We previously determined the crystal structure of the C-terminal 73-residue fragment of PhBCCP (PhBCCPΔN76) that represents the biotinyl(/lipoyl attachment) domain of the hypothetical methylmalonyl-CoA decarboxylase γ chain. This domain adopts a flattened β-barrel comprising two homologous ‘hammerhead’ structures that confer an intramolecular pseudo-twofold symmetry reflecting the gene duplication. In this work, we used the C-terminal 70-residue fragment of PhBCCP (PhBCCPΔN79) as the template to prevent the N-terminal heterogeneity that was observed in PhBCCPΔN76. Moderate deviations of up to 2.53 Å were observed at residues 114–116, which constitute a flexible β-turn harbouring the Lys115 residue to be biotinylated.

In the PhBCCP system (PhBCCPΔN79) residue 138 was selected as the target residue for the mutation experiment because it is a solvent-exposed and nonconserved residue on a surface β-sheet. Moreover, in modelling it could be replaced by any other residue except for proline without intramolecular steric hindrance. Considering the balance of crystal-packing propensity for β-sheet and comparison with the SER method, we designed a systematic site-directed mutagenesis substituting Ala138 with residues of six other types: Ile (the highest crystal-packing propensity), Tyr, Arg, Gln, Val and Lys (the lowest propensity). The isoleucine mutant (A138I) and the tyrosine mutant (A138Y) conferring residue 138 with the highest crystal-packing propensities for β-sheet provided better crystallization scores when compared with other constructs, including the wild type. The A138I mutant and the A138Y mutant produced another orthorhombic crystal form belonging to space group C2221 and a trigonal crystal form belonging to space group P3121, respectively. The crystal structures of the A138I and A138Y mutants were determined at resolutions of 1.9 and 1.5 Å, respectively. In these mutant crystals the crystal-packing interface involving residue 138 differs completely from those of the other two crystal forms. Neither the C orthorhombic nor the trigonal crystals could be obtained with the wild-type protein. Therefore, it is conceivable that the substitution of Ala by Ile/Tyr with a better crystal-packing propensity created novel packing interfaces. On the other hand, the crystal packings of the A138I and A138Y mutants are rich in attractive electrostatic interactions and nonpolar interactions, respectively. In terms of buried ASA, the residue at position 138 in the mutant crystals contributes more to crystal packing when compared with that in the wild-type crystal.

> MENVVSAPMPGKVLRVLVRVGDRVRVGQGLLVLEAMKMENEIPSPRDGVVKRILVKEGEIVDTGQPLIELG>MRGSHHHHHHYVAALFFLIPLVALGFAAANFAAVVRKPEGTERMKEISSYIRSGADSFLAHETKAIFKVAIVIAILLMIFTTWQTGVAFLLGAVMSASAGIVGMKMATRANVRVAEAARTTKKIGPALKVAYQGGSVMGLSVGGFALLGLVLVYLIFGKWMGQVDNLNIYTNWLGINFVPFAMTVSGYALGCSIIAMFDRVGGGVYTKAADMAADLVGKTELNLPEDDPRNPATIADNVGDNVGDVAGLGADLLESFVGAIVSSIILASYMFPIYVQKIGENLVHQVPKETIQALISYPIFFALVGLGCSMLGILYVIVKKPSDNPQRELNISLWTSALLTVVLTAFLTYFYLKDLQGLDVLGFRFGAISPWFSAIIGIFSGILIGFWAEYYTSYRYKPTQFLGKSSIEGTGMVISNGLSLGMKSVFPPTLTLVLGILFADYFAGLYGVAIAALGMLSFVATSVSVDSYGPIADNAGGISEMCELDPEVRKITDHLDAVGNTTAAIGKGFAIGSAIFAALSLFASYMFSQISPSDIGKPPSLVLLLNMLDARVIAGALLGAAITYYFSGYLISAVTKAAMKMVDEIRRQAREIPGLLEGKAKPDYNRCIEITSDNALKQMGYPAFIAILTPLVTGFLLGAEFVGGVLIGTVLSGAMLAILTANSGGAWDNAKKYLEAGNLEGYGKGSEPHKALVIGDTVGDPLKDTVGPSLDILIKIMSVVSVIAVSIFKHVHLF[4x]

Membrane-bound pyrophosphatases (mPPases) facilitate the transport of protons and/or sodium ions across membranes while catalysing the breakdown of pyrophosphate (PPi), a by-product generated in various cellular synthetic reactions – into inorganic phosphate (Pi). Similarly, VrPPase has been solved in multiple states, including IDP-bound (VrPPase:IDP), single phosphate-bound (VrPPase:Pi), two phosphates bound (VrPPase:2Pi), and different mutations at the hydrophobic gate. These structures show that mPPases are homodimeric enzymes, with each monomer consisting of 16 and, as found in sequence databases, occasionally 17 transmembrane helices (TMHs), organised into two concentric rings: the inner ring (TMH5–6, 11–12, and 15–16) and the outer ring (TMH1–4, 7–10, and 13–14). Each monomer consists of four regions: a hydrolytic centre, a coupling funnel, an ion gate, and an exit channel (Tsai et al., 2014). Here, we solved two TmPPase structures in complex with ETD and zoledronate (ZLD) and monitored their conformational ensemble using DEER spectroscopy in solution.

In contrast to the TmPPase:ETD structure, the TmPPase:ZLD structure adopts a partially closed conformation. The overall structure is more similar to the IDP-bound structure (RMSD/Cα of 0.760 Å) than the resting-state structure (RMSD/Cα of 2.32 Å). However, compared to the IDP-bound structure, the TmPPase:ZLD structure exhibits noticeable movements in three of six inner ring helices (TMH11, 12, and 15) and seven of ten outer ring helices (TMH1–4 and 7–9). These movements extend outwards from the hydrolytic centre, leaving it only partially closed. A cross-sectional view confirms this observation, showing the tunnel extending from the hydrolytic centre to the enzyme surface, unlike in the IDP-bound structure, where it is closed. This is because ZLD is sterically bulkier than IDP due to the presence of the heteroaryl group, which points towards TMH11, 12, and 15 on the cytoplasmic side. Although the hydrolytic centre of TmPPase:ZLD is more open, the coordination of the Mg4ZLD complex with the active site residues closely resembles that of Mg5IDP in the IDP-bound structure. ZLD is nonetheless positioned about 1.0 Å above IDP because the steric bulk prevents it from sitting deeper into the hydrolytic centre. However, unlike the IDP-bound structure, and even though the arrangement of TMHs in the ion gate is almost identical, we did not observe any density for a Na+ in the TmPPase:ZLD structure despite its higher resolution (i.e. 3.26 Å compared to 3.5 Å for the IDP-bound structure). In the TmPPase:ZLD structure, D70316.46 and K70716.50 are oriented relatively similarly to the Na+ binding position in the TmPPase:IDP structure, but no Na+ density was observed despite the higher resolution compared to the TmPPase:IDP structure (3.26 Å compared to 3.5 Å for the IDP-bound structure).> GGAGCAUCGUGUCUCAAGUGCUUCACGGUCACAAUAUACCGUUUCGUCGGGUGCGUGGCA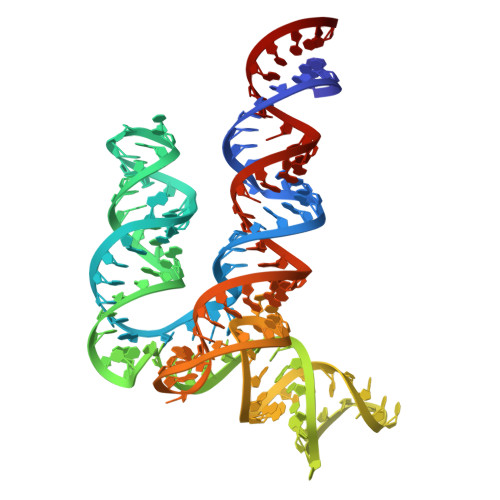AUUCGGUGCACAUCAUGUCUUUCGUGGCUGGUGUGGCUCCUCAAGGUGCGAGGGGCAAGUAUAGAGCAGAGCUCC> GGGLGLIKSLA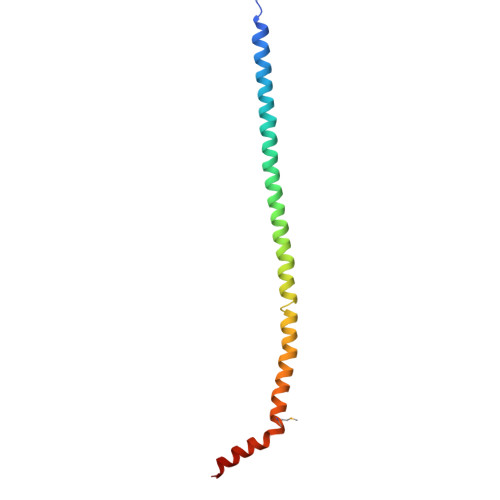EKEKQLLERLEAAKKEAEERVKRAEAEAKALLEEAEAKAKALEAQYRERERAETEALLARYRERAEAEAKAVREKAMARLDEAVALVLKEVLP N4-[2-methoxy-4-[4-(4-methylpiperazin-1-yl)piperidin-1-yl]phenyl]-N2-(2-propan-2-ylsulfonylphenyl)-1,3,5-triazine-2,4-diamine 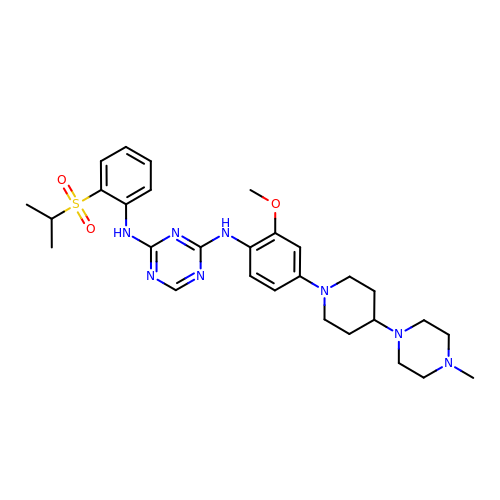| C29 H40 N8 O3 S | MGGBYMDAPCCKCT-UHFFFAOYSA-N>[4x]ESEKIYKVME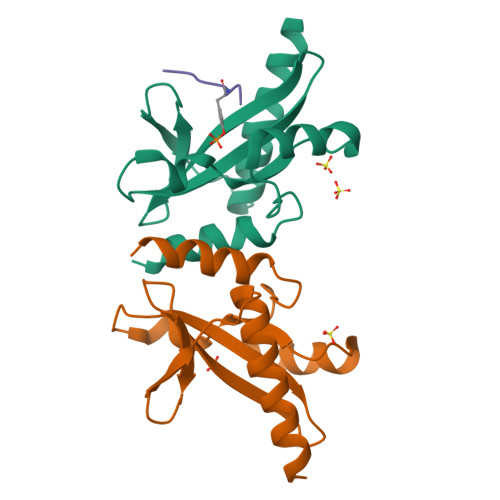EIFVDRHYKENIRTGEEVKQYFSKSKAEFILRWSSANESDTENKYVFIAASFQASDGIHSIRYGINKNGELFSINTASNKVTPIDILPLGVMATLTQHITQNKELIEKAL;>PSYVNVQ[3x]>[2x]APLAATASKFLGCAYGAQQAPGFAQYWNKLTPENGGKWGSVEAVRDQMDWSTLDAAYRFAQANQMPFQMHVMVWGNQQPEWIKTLRPAEQRRE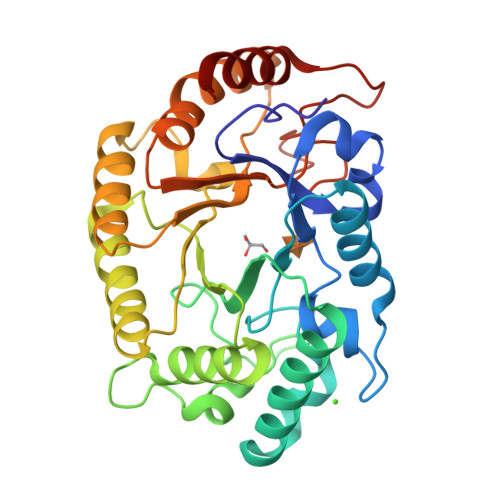IEQWFAAVAQRYPDIALLEVVNEPLNDPPSKADTGGGNYLQALGGNGDSGWEWVLQSFRLARRHFPHTKLMINDYSITSSAQATQKYLQIVRLLQRENLVDAIGVQEHAFETTPEVAVSVHRDNLDALAATGLPIYITEFDLDGPTDAQQLADYKRVFPVFWEHPAVHGITLWGFRPGLWRDKEAAYLIRADGTERPALTWLRDYVAAHP4-[(~{Z})-1-cyano-2-[5-[2-hydroxyethyl(methyl)amino]pyrazin-2-yl]ethenyl]benzenecarbonitrile 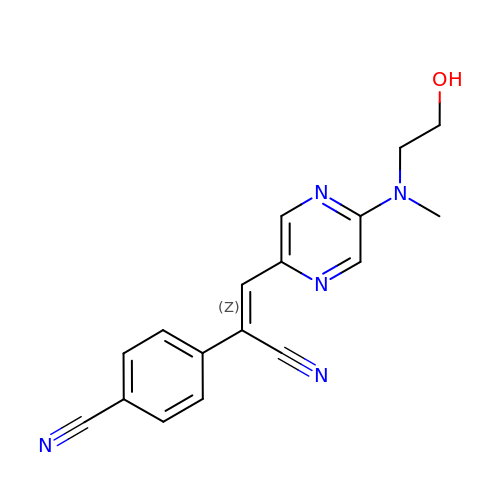| C17 H15 N5 O | KAAHKPAHANCLED-OVCLIPMQSA-N> GGAAUAUCGUCAUGGUGAUUCGUCACCAUGAGGCUAGAUCUCAUAUCUAGCGCUUUCGAGCGCUAGAGUCCUUAUCUAGCCGGUUUAUACUUUCGAGU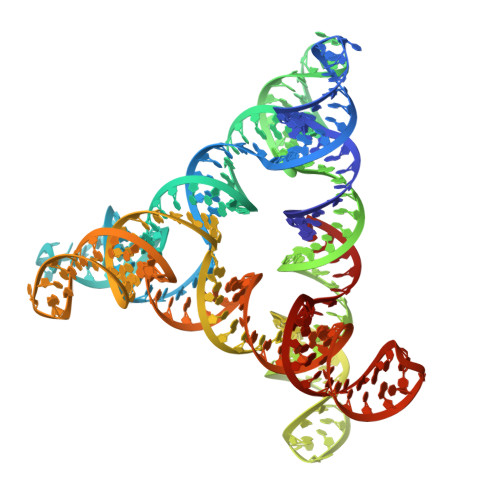GUGAACCCGAUAUUCCGCGGAUCACUAUGAGUCGUUCGCGGCUCAUAGUCCGGCUCAAAGGACAUCAUGGCCUGUUCGCAGGUUGUGAUUAUGAGUGAGCCGGGUAAGGCAUACCGUUCGCGGUAUGUCUUACGAUCCGC> LR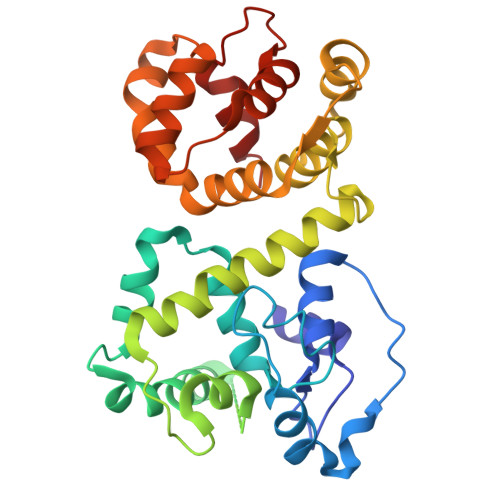KQRFMQFSSLEHEGEYYMTPRDFLFSVMFEQMERKTSVKKLTKKDIEDTLSGIQTAGCGSTFFRDLGDKGLISYTEYLFLLTILTKPHSGFHVAFKMLDTDGNEMIEKREFFKLQKIISKQDDLMTVKTNETGYQEAIVKEPEINTTLQMRFFGKRGQRKLHYKEFRRFMENLQTEIQEMEFLQFSKGLSFMRKEDFAEWLLFFTNTENKDIYWKNVREKLSAGESISLDEFKSFCHFTTHLEDFAIAMQMFSLAHRPVRLAEFKRAVKVATGQELSNNILDTVFKIFDLDGDECLSHEEFLGVLKNR>AALRQPQVAELLAEARRAFREEFGAEPELAVSAPGRVNLIGEHTDYNQGLVLPMALELMTVLVGSPRKDGLVSLLTTSEGADEPQRLQFPLPTAQRSLEPGTPRWANYVKGVIQYYPAAPLPGFSAVVVSSVPLGGGLSSSASLEVATYTFLQQLCPDSGTIAARAQVCQQAEHSFAGMPCGIMDQFISLMGQKGHALLIDCRSLETSLVPLSDPKLAVLITN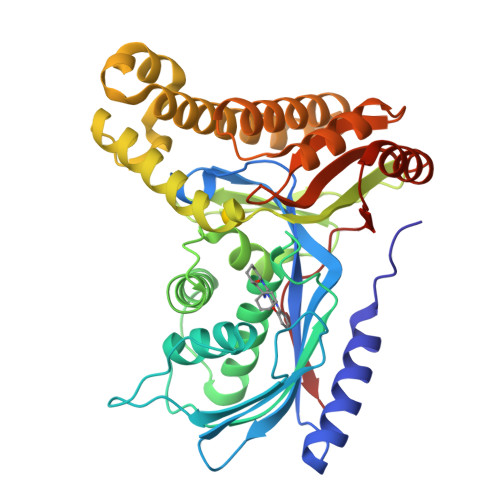SNVRHSLASSEYPVRRRQCEEVARALGAASLREVQLEELEAARDLVSKEGFRRARHVVGEIRRTAQAAAALRRGDYRAFGRLMVESHRSLRDDYEVSCPELDQLVEAALAVPGVYGSRMTGGGFGGCTVTLLEASAAPHAMRHIQEHYGGTATFYLSQAADGAKVLCL[4x]>[2x]SMMQKLVVTRLSPNFREAVTLSRDCPVPLPGDGDLLVRNRFVGVNASDINYSAGRYDPSVKPPFDIGFEGIGEVVALGLSASARYTVGQAVAYMAPGSFAEYTVVPASIATPVPSVKPEYLTLLVSGTTAYISLKELGGLSEGKKVLVTAAAGGTGQFAMQLSKKAKCHVIGTCSSDEKSAFLK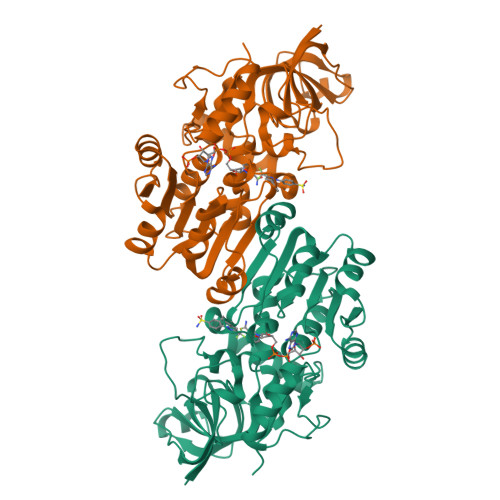SLGCDRPINYKTEPVGTVLKQEYPEGVDVVYESVGGAMFDLAVDALATKGRLIVIGFISGYQTPTGLSPVKAGTLPAKLLKKSASVQGFFLNHYLSKYQAAMSHLLEMCVSGDLVCEVDLGDLSPEGRFTGLESIFRAVNYMYMGKNTGKIVVELPH>MAHHHHHHMNDFHHDFQQQQPTTGIHEEMLKDGIRTNAYKNAILQNKHLFKDKVVLDIGCGTGILCLFAAKAGA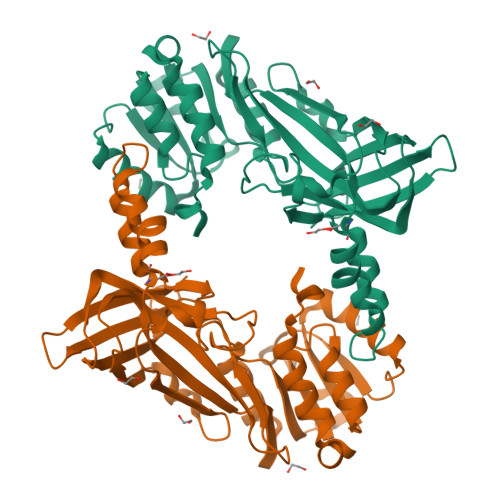KRVIGIDMSDIIDKARQIVSDNGYSHVIELIKGKVEDIAQLPFGIEKVDIIISEWMGYFLLYESMLQTVLSARDRWLRPGGYLFPDKCTMYICGIEDSEYKRDKIDFWDNVYGFNFSAIKADALREPLVDFVESQQIITTQSKFLEIDLNTIQPEDLKQITTSFEFTSQYQEYCQAFVAWFDCVFSRGPHKPVEFSTGPFTEGTHWKQTVFYLENDLPLKPNDVIKGTITISQNKSNHRDLDISMKYTVNGGAVISQDYIMR[6x]>[2x]LSNEKKAKKVRFYRNGDRYFKGIVYAVSSDRFRSFDALL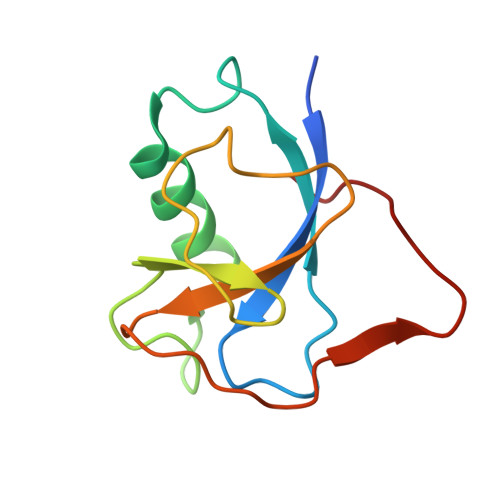ADLTRSLSDNINLPQGVRYIYTIDGSRKIGSMDELEEGESYVCSSDNFFDDVEYTKNVNPNWSVNV> FMVSLPRMVYPQPKVLTPCRKDVLVVTPWLAPIVWEGTFNIDILNEQFRLQNTTIGLTVFAIKKYVAFLKLFLETAEKHFMVGHRVHYYVFTDQPAAVPRVTLGTGRQLSVLEVGAYKRWQDVS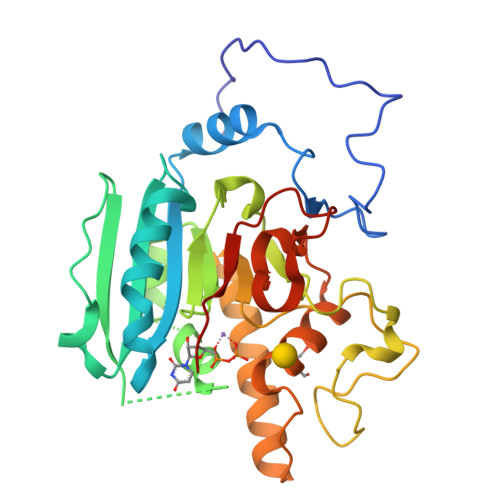MRRMEMISDFCERRFLSEVDYLVCVDVDMEFRDHVGVEILTPLFGTLHPSFYGSSREAFTYERRPQSQAYIPKDEGDFYYMGAFFGGSVQEVQRLTRACHQAMMVDQANGIEAVWHDESHLNKYLLRHKPTKVLSPEYLWDQQLLGWPAVLRKLRFTAVPKNHQAVRNP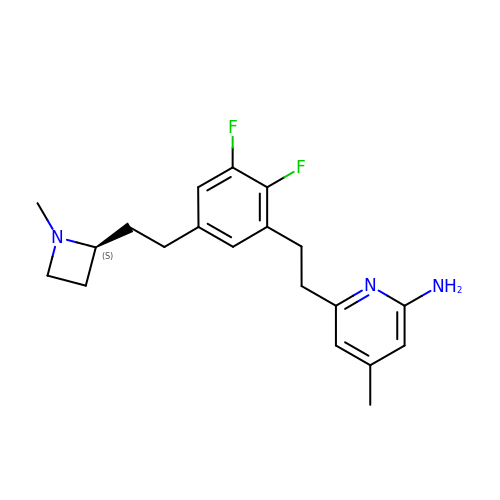6-[2-(2,3-difluoro-5-{2-[(2S)-1-methylazetidin-2-yl]ethyl}phenyl)ethyl]-4-methylpyridin-2-amine | C20 H25 F2 N3 | STGWAFUVRUKRNW-KRWDZBQOSA-N>[2x]TGSTGSTGSTGSQQKRAFEYEIRFYTGNDPLDVWDRYISWTEQNYPQGGKESNMSTLLERAVEALQGEKRYYSDPRFLNLWLKLGRLCNEPLDMYSYLHNQGIGVSL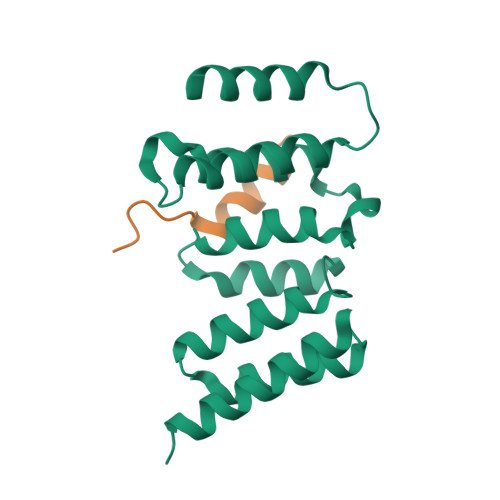AQFYISWAEEYEARENFRKADAIFQEGIQQKAEPLERLQSQHRQFQARVSRQTLLALEKEEEEEVFESS;>GPLGSSSENKIDFNDFIKRLKTGK[2x]> MSFVKDFKPQALGDTNLFKPIKIGNNELLHRAVIPPLTRMRALHPGNIPNRDWAVEYYTQRAQRPGTMIITEGAFISPQAGGYDNAPGVWSEEQMVEWTKIFNAIHEKKSFVWVQLWVLGWAAFPDNLARDGLRYDSASDNVFMDAEQEAKAKKANNPQHSLTKDEIKQYIKEYVQAAKNSIAAGADGVEIHSANGYLLNQFLDPHSNTRTDEYGGSIENRARFTLEVVDALVEAIGHEKVGLRLSPYGVFNSMSGGAETGIVAQYAYVAGELEKRAKAGKRLAFVHLVEPRVTNPFLTEGEGEYEGGSNDFVYSIWKGPVIRAGNFALHPEVVREEVKDKRTLIGYGRFFISNPDLVDRLEKGLPLNKYDRDTFYQMS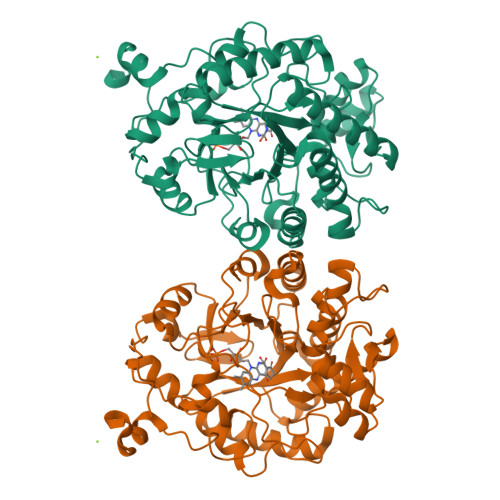AHGYIDYPTYEEALKLGWDKK> MSKKSGKGKGKNDGDELGAEKEQVLRTKVESLIQRLGHEQERADRAKAAENELRARLFDLDKDFKNEKDRLFSITSDMTRQYKQMQDELLNQVNDLNKTVIEK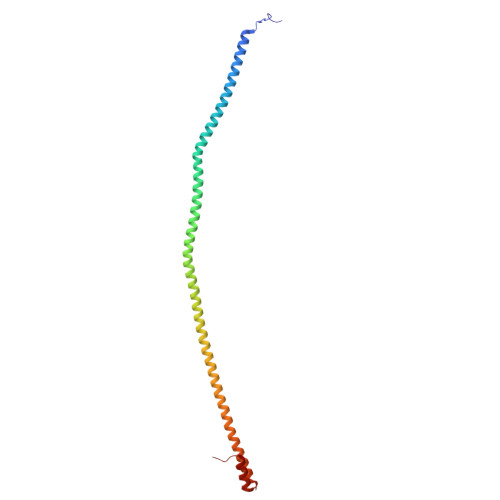DEEIKKKDQQIQDMTKDYEYKLKKKDDEIQDLKRKIEEMSAEFAKMLKDTLDKMQERIEMVQWDSDTDPQMMKRLKDMTGLSNN>HHHHFNLPPGNYKKPKLLYCSNGGHFLRILPDGTVDGTRDRSDQHIQLQLSAESVGEVYIKSTETGQYLAMDTDGLLYGSQTPNEECLFLERLEENHYNTYISKKHAEKNWFVGIKKNGSCKRGPRTHYGQKAILFL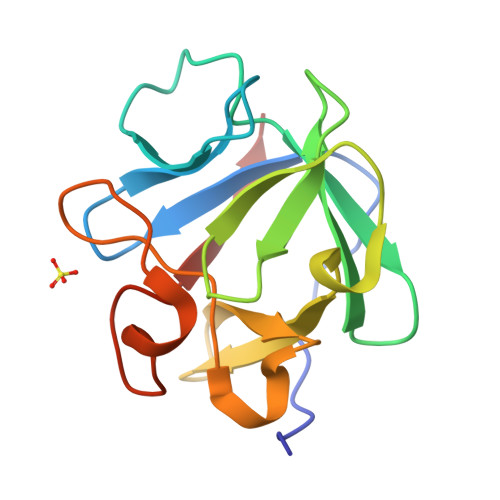PLPVSSD[2x]>[2x]GAMALPQGDEIAYVPIGSITLESGAVIDDVTIAVQSWGELSPRRDNVVFVCHALTADSHVVGPAGPDHITGGWWEGIIGPGAAIDTDHWCAVATNVLGGCRGTTGPTSLARDGKPWGSRFPEVSVRDQVNADVAALAQLGITEVAAVVGGSMGGARALEWAVMHPDAVRAALVLAVGARATGDQIGTQSTQIAAIQTDPDWQGGDYHGSGRSPGKGLNLARRIAHLTYRGEVELDTRFGNDPQVGPDGPEDPWADGRYAVQSYLEHQGNKFVRRFDAGSYVILTESLNRHDVGRGRGGVEKALRGCPVPVVVGGITSDRLYPLRLQEELADLLPGCTGLRVVESVHGHDAFLIEFDAVSELVRETLALAK

MetX (previously mis-annotated as MetA in the reference genome of M. tuberculosis) is an l-homoserine O-acetyltransferase, commonly also referred to as a homoserine transacetylase (HTA) and is a crucial enzyme in the biosynthesis of methionine and threonine. Here we report the structures of three homologous MetX enzymes from Mycobacterium tuberculosis (MtMetX), Mycolicibacterium abscessus (MaMetX), and Mycolicibacterium hassiacum (MhMetX) and compare them to previously solved structures of HTAs in order to begin development of selective inhibitors of MtMetX via a structure-based approach. Two copies of each monomer exist in the asymmetric unit of all three structures. MetX can be divided into two distinct structural domains, the catalytic domain, and the lid domain. The organization of the catalytic domains’ fold marks MetX as members of the α/β-hydrolase super-family.

The three solved MetX structures include residues 15–70, 77–372 from MhMetX, 10–379 from MaMetX, and 7–372 from MtMetX. The catalytic domain comprises residues 15–181, 297–372 of MhMetX, residues 17–183, 304–379 of MaMetX and residues 17–181, 311–372 of MtMetX. For MtHTA and MhHTA, Ser157, Asp320, and His350 comprise the active site; MaHTA’s triad is comprised of Ser160, Asp327, His357. MtMetX and MsHTA both contain a small helical region (αL1′); MaHTA features a unique pair of short anti-parallel sheets (β1′, β2′). Temperature factors of the equivalent rings in MhMetX is B = 19 Å2, while both MtMetX and MaMetX are B = 21 Å2, values very similar to the HiHTA structure with B = 16 Å2. MaMetX shows a similar pattern with the top clusters appearing nearly overtop those of MtMetX with S = 26, S = 13 and S = 10. M. abscessus MetX was initially chosen for study due to its high similarity to the Mtb variant. However, the structure and CS data argue that it might make an excellent secondary target for drug development. Many compounds that inhibit MtMetX are also likely to affect MaMetX. M. abscessus is an emerging public-health threat, primarily implicated in pulmonary infections.> NECLG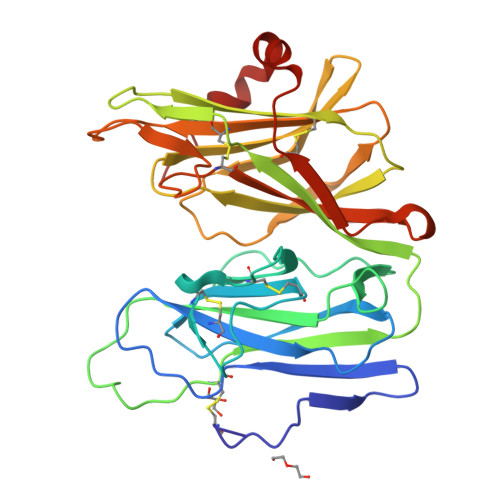TIGPVTPLDASDFALDIRMPGVTPKESDTYFCMSMRLPVDEEAFVIDFKPRASMDTVHHMLLFGCNMPSSTGSYWFCDEGTCTDKANILYAWARNAPPTRLPKGVGFRVGGETGSKYFVLQVHYGDISAFRDNHKDCSGVSVHLTRVPQPLIAGMYLMMSVDTVIPPGEKVVNADISCQYKMYPMHVFAYRVHTHHLGKVVSGYRVRNGQWTLIGRQNPQLPQAFYPVEHPVDVTFGDILAARCVFTGEGRTEATHIGGTSSDEMCNLYIMYYMEAKYALSFMTCTKNVAPDMFRTIPAEANIPIPV4-(aminomethyl)-~{N}-(pyridin-2-ylmethyl)benzenesulfonamide 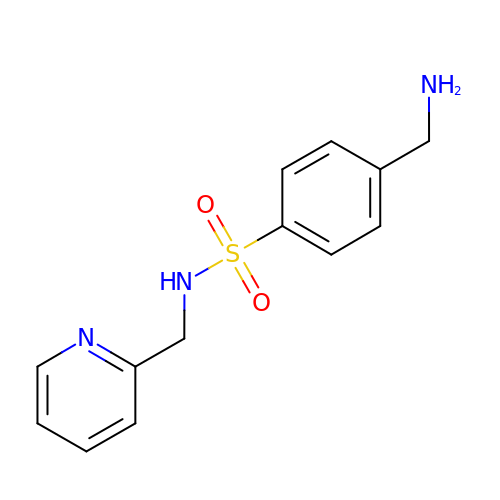| C13 H15 N3 O2 S | XVNHUDOTGRKSHU-UHFFFAOYSA-N>SKTKPFTLPILTISELTNSRFPIPIE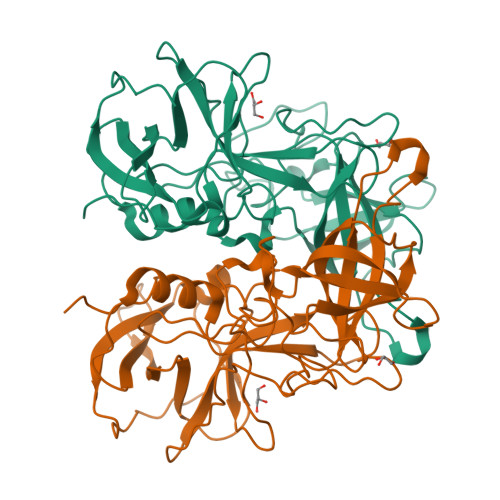QLYTAPNENNVVQCQNGRCTLDGELQGTTQLLSSAVCSYRGRTVANSGDNWDQNLLQLTYPSGASYDPTDEVPAPLGTQDFRGILYGVLTQDNVSEGTGEAKNAKGVYISTTSGKFTPKIGSIGLHSITENVHPNQQSRFTPVGVAQNENTPFQQWVLPHYAGALALNTNLAPAVAPTFPGEQLLFFRSRVPCVQGLRGQDAFIDCLLPQEWVNHFYQEAAPSQADVALIRYVNPDTGRTLFEAKLHRSGFITVSHTGAYPLVVPPNGHFRFDSWVNQFYSLAPMGTGNGR[2x]> MYTAYPYPKGKTYVYDNRYWKNLGGVIKNAKRRKHEEEQEKVEREFDSLDKYLVAEDPFCGPGKNQKLTLFKEIRNIKPDTMKLIVNWSGKEFLRETWTRFMEDSFPIVNDQEVMDVFLVINMR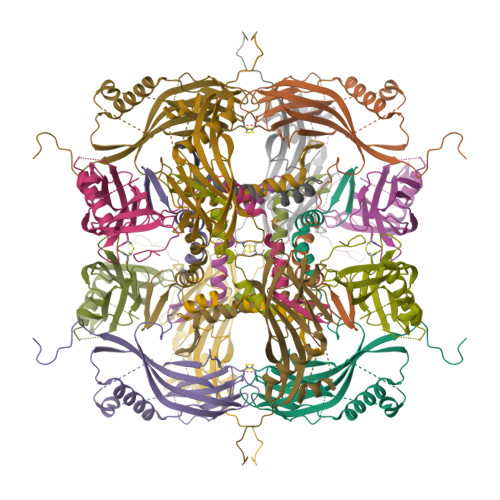STKPNRCFRFLAQHALRCDPDYVPHEIIRIVEPSYVGNNEYRISLAKRGGGCPIMNLHLEYTNSFEHFINKVIWENFYKPIVYIGTDSAEDEEVLFEVSLVFKIKEFAPDAPLFSGPAY> GMSSTSSKVVLHPTMLNCMRGLHKKAVLPEPVLDRGIELARAFVGGRRARGQRVERQPDVAAACLMIAAEEAQQPLPLAEVRCLDSSLGDVELRRADIVRELHLEDSERRLRDTFADNLLVKYILKLGLQVSLYLPHCKRLLTALGRVEALAG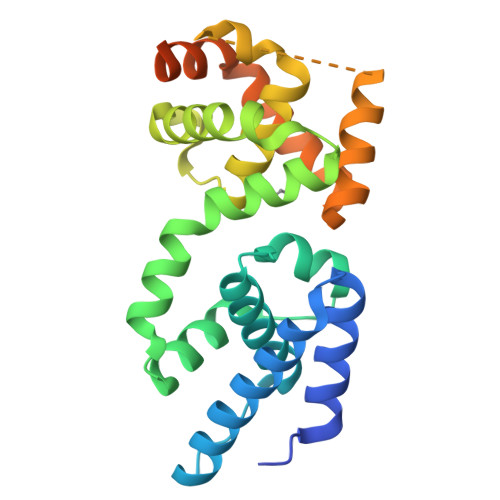LTVADRVTTALLLARTAQTLSWEQGTHISKGKECDLGMEAIYANFSSKAHLEVTKVNKIMHLAVDVLPLIQAAFQDCGEPTAGKRKVDKNSEPEASGGTKRVKREET>MKFSNITIKNFRNFEKVNINLDNKNVIFGMNDIGKTNFLYALRFLLDKEIRKFGFNKSDYHKHDTSKKIEIILTLDLSNYEKDEDTKKLISVVKGARTSANADVFYIALESKYDDKELYGNIILKWGSELDNLIDIPGRGNINALDNVFKVIYINPLVDLDKLFAQNKKYIFEESQGNESDEGILNNIKSLTDQVNQQIGEMTIIKGFQQEITSEYRSLKKEEVSIELKSEMAIKGFFSDIIPYIKKDGDSNYYPTSGDGRRKMLSYSIYNYLAKKKYEDKIVIYLIEEPEISLHRSMQIALSKQLFEQSTYKYFFLSTHSPELLYEMDNTRLIRVHSTEKVVCSSHMYNVEEAYGSVKKKLNKALSSALFAERVLLIEGPSEKILFEKVLDEVEPEYELNGGFLLEVGGTYFNHYVCTLNDLGITHIIKTDNDLKSKKGKKGVYELLGLNRCLNLLGRENLDEITIDIPEDIKGKKKKERLNERKKEIFKQYKNEVGEFLGERIYLSEIDLENDLYSAIGESMKRIFENEDPVHYLQKSKLFNMVELVNNLSTKDCFDVFEHEKFACLKELVGSDRG[4x];>MSREQIIKDGGNILVTAGAGSGKTTILVSKIEADLKENKTHYSIAAVTFTNKAAKEIEGR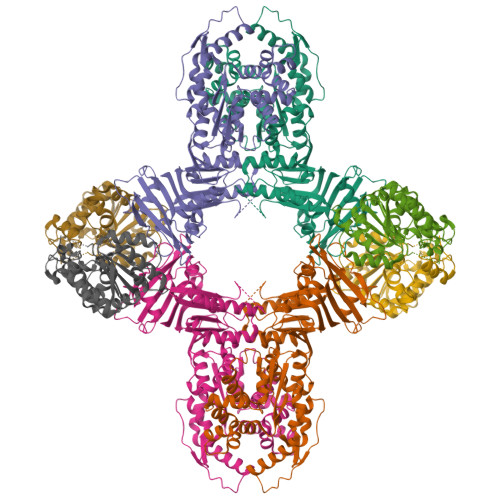LGYSSRGNFIGTNDGFVESEIIRPFIKDAFGNDYPDNFTAEYFDNQFASYDKGLQVLKYQNILGTYSNPKKNFKFQLALDILKKSLVARQYIFSKYFKIFIDEYQDSDKDMHNLFMYLKDQLKIKLFIVGDPKQSIYIWRGAEPENFNGLIENSTDFNKYHLTSNFRCCQDIQNYSNLFNEETRSLIKEKNEVQNVISIADDMPISDILLKLTEEKQVLNIEAELVILVRRRNQAIEIMKELNEEGFNFIFIPQTPLDRATPNATLLKEVIKYVKNDRYSIYDLAAEIVGNLSSREIKEIQKIINELLVPNINQVLINQVLINLFAKLEITLDTREITAFTEVMMTNEFDIAFDTNEYLHKIFTVHSAKGLEFNQVIITASDYNVHYNRDTNEHYVATTRAKDKLIVIMDNKKYSDYIETLMKELKIKNIIKSI[4x]>[2x]DWIWNRMHIREEIDSPLPHHVGKLTSSVGNKNAMYIIEGESANTIFKVQGYDGDIYAFERLDREKKAEYELTAHIID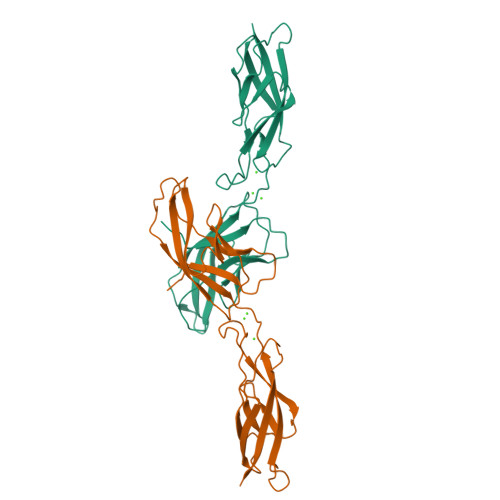RRNNRSLEPPSKFIIKVSDINDNAPIFVQKIFNGSVPEMSRLGTSVTKVTAEDADDPTVAGHATVTYQIIKGNEYFTVDDSGVIFTARADLDRESQSAYEIIVKAKDALGLTGESSTATVIIRLTD> PRKKRPEDFKFGKILGEGSFSTVVLARELATSREYAIKILEKRHIIKENKVPYVTRERDVMSRLDHPFFVKLYFTFQDDEKLYFGLSYAKNGELLKYIRKIGSFDETCTRFYTAEIVSALEYLHGKGIIHRDLKPENILLNEDMHIQITDFGTAKVLSPESKQARANSFVGTAQYVSPELLTEKSACKSSDLWALGCIIYQLVAGLPPFRAGNEYLIFQKIIKLEYDFPEKFFP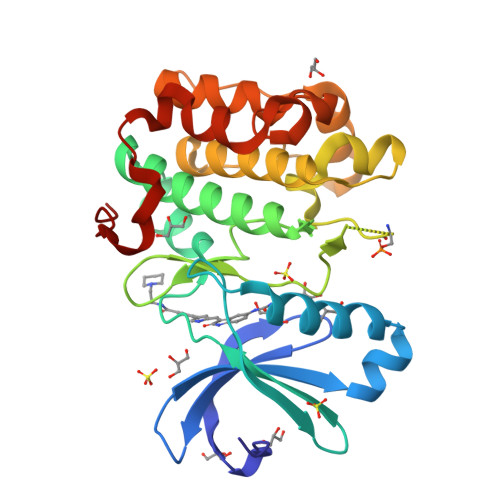KARDLVEKLLVLDATKRLGCEEMEGYGPLKAHPFFESVTWENLHQQTPPKLT> ELHGILSLGLNVDHTIVRKKSIPLFEIGNSDQVCNWIIQIIEAGVDLQEVADSFLTMLCVNHAYQGDPNLFLESPAAHYLKGHGIHFEIQHRDNVDHITDLLGVGSRDKSLRKTLSALEFEPGGTTTAGMFLSFASLFLPKLVVGERACLEKVQRQIQIHAEQGLIQYPTQWQSVGHMMVVFRLIRVNFVLKFLLVHQGMHMMAGHDANDAIIANSISQTRFSGLLIVKTVLEHILQKTEAGVQLHPLARTSKVKGELLAFKSALEALASHREYAPFARLLNLSGVNNLEHGLYPQLSAIALGVATAHGSTLAG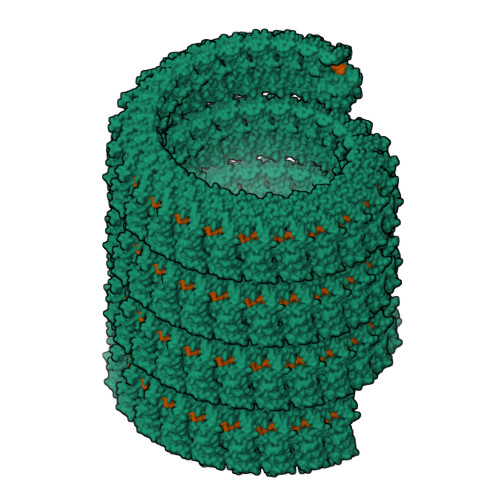VNVSEQYQQLREAATEAEKQLQQHSEMRELETLGLDEQERKILATFHSRKNEINIQQTSSILAIRKERLRKLT>MGSKSFLTEQQIKILRLRARGLKQSEIAELLGTSRANISILERRALEKIEKARNIITIWEQINSKISVEVRKGEDIFTVPDKLFKKADELQIKVPYSTAEIIAFLVEHAPISDRIAKRDFTLFLDARDRLRISECLLEEFDEIGKQHHHHHH[2x]

Thermococcus onnurineus NA1, a hyperthermophilic carboxydotrophic archaeon, produces H2 through CO oxidation catalyzed by proteins encoded in a carbon monoxide dehydrogenase (CODH) gene cluster. TON_1525 with a DNA-binding helix-turn-helix (HTH) motif is a putative repressor regulating the transcriptional expression of the codh gene cluster. Monomeric TON_1525 adopts a novel ‘eighth note’ symbol-like fold (referred to as ‘eighth note’ fold regulator, EnfR), and the dimerization mode of EnfR is unique in that it has no resemblance to structures in the Protein Data Bank. According to footprinting and gel shift assays, dimeric EnfR binds to a 36-bp pseudo-palindromic inverted repeat in the promoter region of the codh gene cluster, which is supported by an in silico EnfR/DNA complex model and mutational studies revealing the implication of N-terminal loops as well as HTH motifs in DNA recognition.

The T55I mutation in TON_1525 led to enhanced H2 production accompanied by the increased expression of genes in the codh cluster. The KD values of the wild-type and the T55I mutant were calculated to be 61.8 ± 20.5 and 948.0 ± 130.0 nM, respectively, clearly indicating that the DNA-binding affinity of the mutant is much lower (over fifteen-fold) than that of the wild-type. To get structural insights into the reduced DNA-binding activity of the T55I mutant, we determined its 3.4 Å resolution crystal structure. The overall structures of the monomeric and dimeric T55I mutant are virtually identical to those of the wide-type. The r.m.s. deviations of monomers and dimers between the mutant and the wild-type are 0.827 and 0.941 Å, respectively, for all Cα atoms. Despite this structural resemblance, however, the T55I mutant has a remarkable structural difference in the orientation and conformation of the N-6 region that is engaged in DNA recognition. In contrast, in the case of the T55I mutant, the N-6 region runs in a different direction due to the loss of the hydrogen bond, which is the consequence of the isoleucine replacement at position 55. In this conformation of the two N-6 regions, the two phenylalanine residues cannot form π–π stacking interactions. In the resulting complex model, it was obvious that the N-6 region of the mutant clashes with DNA. Consequently, it can be concluded that the altered conformation of the N-6 region induced by the T55I mutation disturbs the DNA-binding activity of the mutant, and the conformation of T55I mutant is not adequate in DNA-binding.> GENIVFRVISTTGQIPIRDFSADISQVL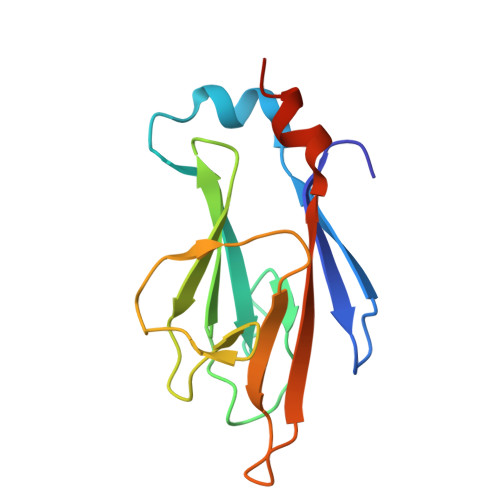KEKRSIKKVWTFGRNPACDYHLGNILPVSNKHFQILLGEDGNLLLNDISTNGTWLNGQKVEKNSYQLLSQGDEITVRTDPTGTILSLVIFINDKFKQSLEQNKVDR>[2x]DVSGTVCLSALPPEA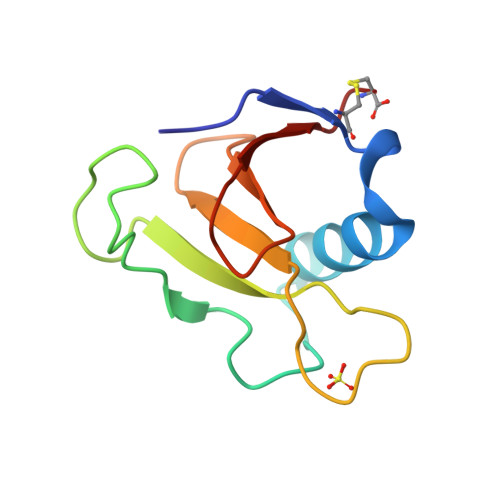TDTLNLIASDGPFPYSQDGVVFQNRESVLPTQSYGYYHEYTVITPGARTRGTRRIITGEATQEDYWTGDHYATFSLIDQTC> MYLTLQEWNARQRRPRSLETVRRWVRESRIFPPPVKDG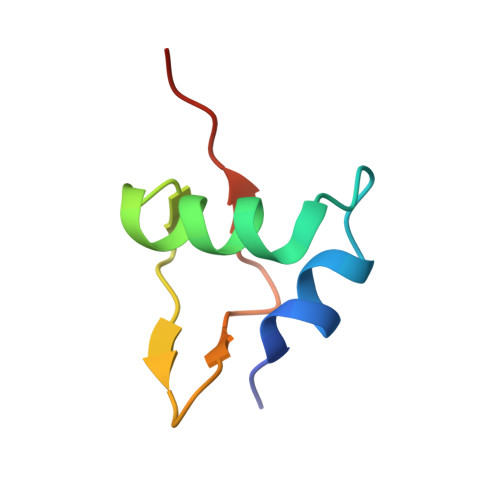REYLFHESAVKVDLNRP> SKGKKRSGARPGRPQPLRGTKGKRKG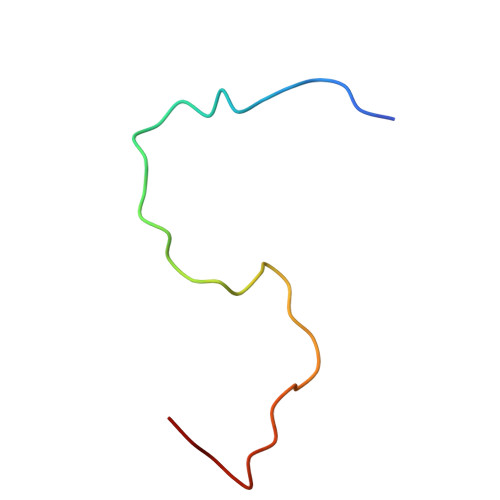ARLWYVGGQQF>[4x]AHMNEIDNGIKALDPFNFYRIRTFCGKMLDVVGQS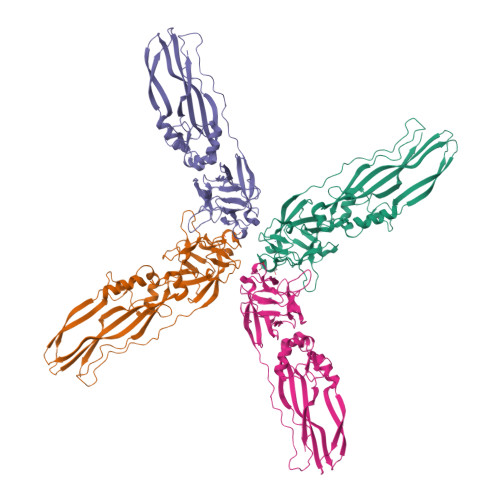TSDNAMVVQYSINNKPNQNFLVFTLDDGYSIIAAENSGKVLDISEDFFFKGMLIQYHFANSDNQKFLISNNGTIAVKRSGKVFDIPGASTSNDAPVIAYNFNNAANQKFTFERVKTFQVPSPSIGTLPPAPDFKNDINEQLPDKTNPVITHFSTIPYIMANDATFNSHQQIQYSPYYKLVRIQYWEKVTQRILGPRDDYEYNKTKGISKTDQVSMTETVSMSVGADFGFMFKGFSASLSAQITKELSVTKSTSTTEMTEETYKEKYTNPFNYELARAQYMLVNEFYVTRMDGTRITANWTLRDNTQTVTRIFPKS>[2x]SM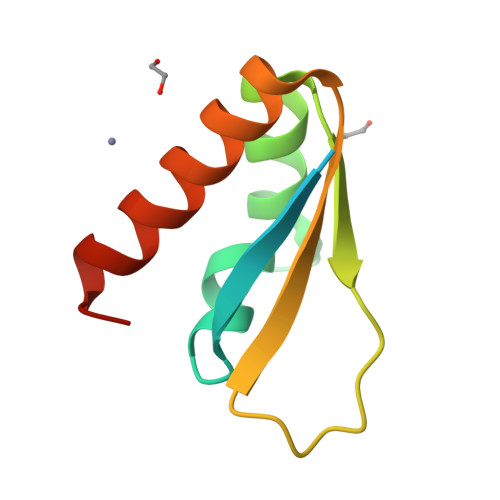FREVRNEYGSRIGGNEGIDVPIPRFAVGIVIGRNGEMIKKIQNDAGVRIQFKPDDGTTPERIAQITGPPDRCQHAAEIITDLLRSVQAGNP>GPGSMRRVVITGLGLVSPLAGDVEYSWKRLLEGKSGVRRITEFDVSDLSCQIAARIPVGDGTNGTYNADLHMESKEQRKVDAFIVYAIAAADQALADAEWFPKSDEDQICTGVLIGSGIGGIEGIVEAGYTLRDKGPRRISPFFIPGRLINLASGYVSIKYGLRGPNHSVVTACSTGAHAIGDAARLIALGDADVMLAGGTESPINRISLAGFSACRALSTCRNDDPERASRPYDVDRDGFVMGEGAAIVVLEELEHAKKRGARIYAEIIGYGLSGDAYHITAPSESGEGAQRSMMAALKRAQVNVSELDYINAHGTSTMADVIELAAVERVLGYYAPQVSMSSTKSSIGHLLGAAGAAEAIF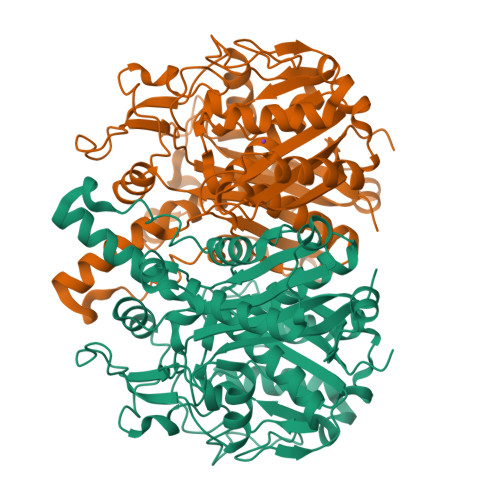CVLAIRDNIAPATLNLENPSIETKIDLVPHKPRERKIDTVLSNSFGFGGTNASLVMRRFSE[2x]> STGSKQRSQNRSKTPKNQEALRMANVAENSSSDQRQACKKHELYVSFRDLGWQDWIIAPEGYAAYYCEGECAFPLNSYMNATNHAIVQTLVHFINPETVPKPCCAPTQLNAISVLYFDDSSNVILKKYRNMVVRACGCH;> AILGRSETQECLFFNANWERDRTNQTGVEPCYGDKDKRRHCFATW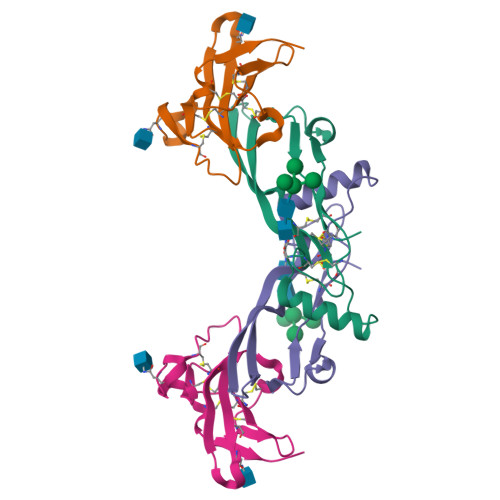KNISGSIEIVKQGCWLDDINCYDRTDCIEKKDSPEVYFCCCEGNMCNEKFSYFPEME>[9x]MEDINFASLAPRHGSRPFMGNWQDIGTSNMSGGAFSWGSLWSGIKNFGSTVKNYGSKAWNSSTGQMLRDKLKEQNFQQKVVDGLASGISGVVDLANQAVQNKINSKLDPRPPVEEPPPAVETVSPEGRGEKRPRPDREETLVTQIDEPPSYEEALKQGLPTTRPIAPMATGVLGQHTPVTLDLPPPADTQQKPVLPGPTAVVVTRPSRASLRRAASGPRSLRPVASGNWQSTLNSIVGLGVQSLKRRRCF;>[12x]MATPSMMPQWSYMHISGQDASEYLSPGLVQFARATETYFSLNNKFRNPTVAPTHDVTTDRSQRLTLRFIPVDREDTAYSYKARFTLAVGDNRVLDMASTYFDIRGVLDRGPTFKPYSGTAYNALAPKGAPNPCEWDEAATALEINLEEEDDDNEDEVDEQAEQQKTHVFGQAPYSGINITKEGIQIGVEGQTPKYADKTFQPEPQIGESQWYETEINHAAGRVLKKTTPMKPCYGSYAKPTNENGGQGILVKQQNGKLESQVEMQFFSTTEATAGNGDNLTPKVVLYSEDVDIETPDTHISYMPTIKEGNSRELMGQQSMPNRPNYIAFRDNFIGLMYYNSTGNMGVLAGQASQLNAVVDLQDRNTELSYQLLLDSIGDRTRYFSMWNQAVDSYDPDVRIIENHGTEDELPNYCFPLGGVINTETLTKVKPKTGQENGWEKDATEFSDKNEIRVGNNFAMEINLNANLWRNFLYSNIALYLPDKLKYSPSNVKISDNPNTYDYMNKRVVAPGLVDCYINLGARWSLDYMDNVNPFNHHRNAGLRYRSMLLGNGRYVPFHIQVPQKFFAIKNLLLLPGSYTYEWNFRKDVNMVLQSSLGNDLRVDGASIKFDSICLYATFFPMAHNTASTLEAMLRNDTNDQSFNDYLSAANMLYPIPANATNVPISIPSRNWAAFRGWAFTRLKTKETPSLGSGYDPYYTYSGSIPYLDGTFYLNHTFKKVAITFDSSVSWPGNDRLLTPNEFEIKRSVDGEGYNVAQCNMTKDWFLVQMLANYNIGYQGFYIPESYKDRMYSFFRNFQPMSRQVVDDTKYKDYQQVGILHQHNNSGFVGYLAPTMREGQAYPANFPYPLIGKTAVDSITQKKFLCDRTLWRIPFSSNFMSMGALTDLGQNLLYANSAHALDMTFEVDPMDEPTLLYVLFEVFDVVRVHRPHRGVIETVYLRTPFSAGNATT;> MMQDATDPAVRAALQSQPSGLNSTDDWRQVMDRIMSLTARNPDAFRQQPQANRLSAILEAVVPARANPTHEKVLAIVNALAENRAIRPDEAGLVYDALLQRVARYNSGNVQTNLDRLVGDVREAVAQRERAQQQGNLGSMVALNAFLSTQPANVPRGQEDYTNFVSALRLMVTETPQSEVYQSGPDYFFQTSRQGLQTVNLSQAFKNLQGLWGVRAPTGDRATVSSLLTPNSRLLLLLIAPFTDSGSVSRDTYLGHLLTLYREAIGQAHVDEHTFQEITSVSRALGQEDTGSLEATLNYLLT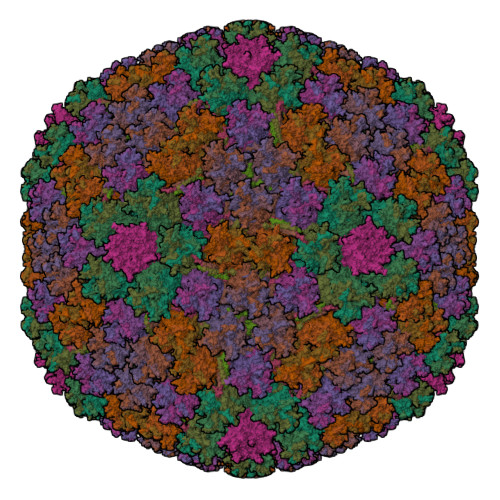NRRQKIPSLHSLNSEEERILRYVQQSVSLNLMRDGVTPSVALDMTARNMEPGMYASNRPFINRLMDYLHRAAAVNPEYFTNAILNPHWLPPPGFYTGGFEVPEGNDGFLWDDIDDSVFSPQPQTLLELQQREQAEAALRKESFRRPSSLSDLGAAAPRSDASSPFPSLIGSLTSTRTTRPRLLGEEEYLNNSLLQPQREKNLPPAFPNNGIESLVDKMSRWKTYAQEHRDVPGPRPPTRRQRHDRQRGLVWEDDDSADDSSVLDLGGSGNPFAHLRPRLGRMF;> MRRAAMYEEGPPPSYESVVSAAPVAAALGSPFDAPLDPPFVPPRYLRPTGGRNSIRYSELAPLFDTTRVYLVDNKSTDVASLNYQNDHSNFLTTVIQNNDYSPGEASTQTINLDDRSHWGGDLKTILHTNMPNVNEFMFTNKFKARVMVSRLPTKDNQVELKYEWVEFTLPEGNYSETMTIDLMNNAIVEHYLKVGRQNGVLESDIGVKFDTRNFRLGFDPVTGLVMPGVYTNEAFHPDIILLPGCGVDFTHSRLSNLLGIRKRQPFQEGFRITYDDLEGGNIPALLDVDAYQASLKDDTEQGGGGAGGSNSSGSGAEENSNAAAAAMQPVEDMNDHAIRGDTFATRAEEKRAEAEAAAEAAAPAAQPEVEKPQKKPVIKPLTEDSKKRSYNLISNDSTFTQYRSWYLAYNYGDPQTGIRSWTLLCTPDVTCGSEQVYWSLPDMMQDPVTFRSTRQISNFPVVGAELLPVHSKSFYNDQAVYSQLIRQFTSLTHVFNRFPENQILARPPAPTITTVSENVPALTDHGTLPLRNSIGGVQRVTITDARRRTCPYVYKALGIVSPRVLSSRTF;>[4x]MSTNSFDGSIVSSYLTTRMPPWAGVRQNVMGSSIDGRPVLPANSTTLTYETVSGTPLETAASAAASAAAATARGIVTDFAFLSPLASSAASRSSARDDKLTALLAQLDSLTRELNVVSQQLLDLRQQVSALKASSPPNAV;>MSKEIPTPYMWSYQPQMGLAAGAAQDYSTRINYMSAGPHMISRVNGIRAHRNRILLEQAAITTTPRNNLNPRSWPAALVYQESPAPTTVVLPRDAQAEVQMTNSGAQLAGGFRHRVRSPGQGITHLTIRGRGIQLNDESVSSSLGLRPDGTFQIGGAGRPSFTPRQAILTLQTSSSEPRSGGIGTLQFIEEFVPSVYFNPFSGPPGHYPDQFIPNFDAVKDSADGYD[2x]>[3x]TRDQNGTWEMESNENFEGYMKA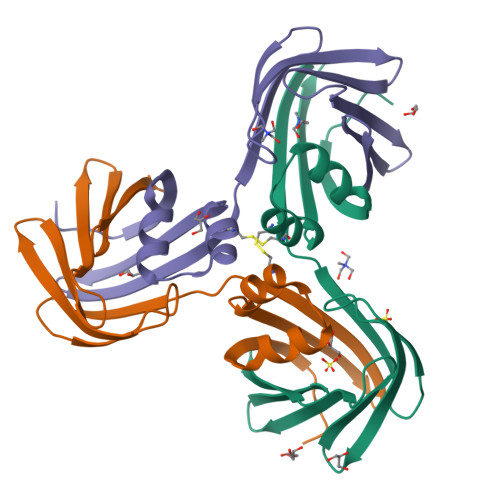LDIDFCTRKCAVRLTQTKVIDQDGDNFKDKTTSTFRNYDVDFTVGVEFDEYTKSLDNRHVKALVTWEGDVLVCVQKGEKENRGWKKWIEGDKLYLELTCGDQVCRQVFKKK>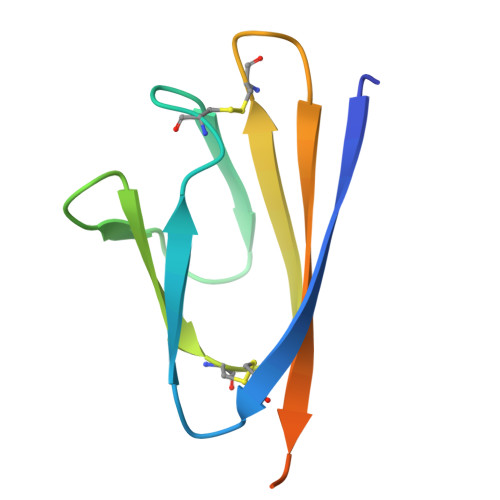 MTCELYHYQECVRGTTVLLKEPCSSGTYEGNSPFHPLADNKFALTCFSTQFAFACPDGVKHVYQLRARSVSPKLFIRQEEVQEL> KPDFCFLEEDPGICRGYITRYFYNNQTKQC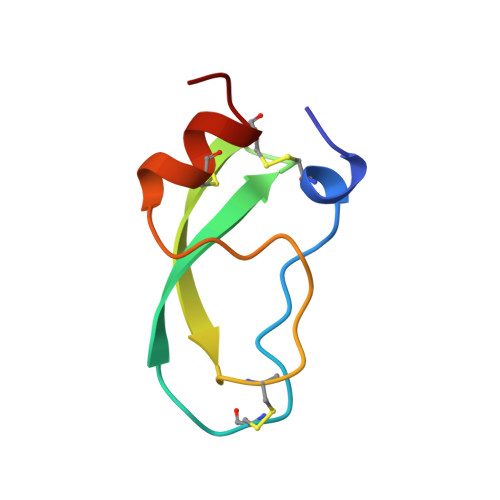ERFKYGGCLGNMNNFETLEECKNICEDG> GPLGSEQKKMKYLENLVGKTPMLELIFDYKGEERRIFVKNESYNLTGSIKDRMAFYTLKKAYEKNEIKKGAPIVEATSGNTGIAFSAMGAILGHPVIIYMPDWMSEERKSLIRSFGAKIILVSRKEGGFLGSIEKTKEFAKNNPDTYLPSQFSNLYNSEAHYYGIGLEIVNEMKSLNLNIDGFVAGVGTGGTVMGIGKRIKENFSNAKICPLEPLNSPTLSTGYKVAKHRIEGISDEFIPDL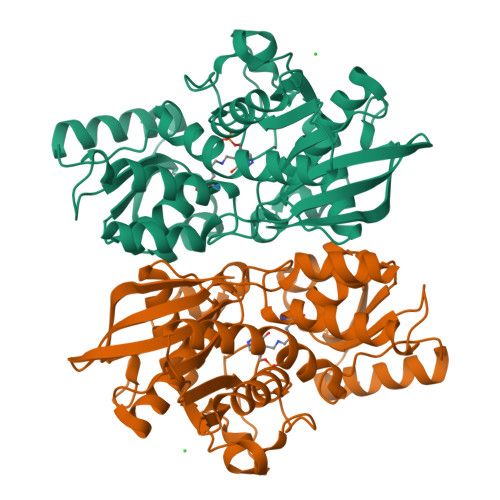VKLDKLDNVVSVDDGDAIVMAQKLAKCGLGVGISSGANFIGALMLQNKLGKDSVIVTVFPDDNKKYLSTDLMREEKVKEDFLSKDITLKEIKNVLRVI The male abnormal 21 (MAB21) like proteins form a sequence related subfamily within the large and diverse family of nucleotidyltransferase (NTase) fold proteins. Here, we provide the first crystal structure of a MAB21 protein and the structure of MAB21L1 bound to CTP. MAB21L1 is a two lobed, globular protein of a mixed α/β topology with approximate molecular dimensions of 64 Å × 35 Å × 48 Å. The human MAB21L1 structure exhibits a high degree of structural conservation with cGAS but features a number of differences.

We crystallized native MAB21L1 in space group C2 with unit cell constants a = 167.7 Å, b = 177.6 Å, c = 115.6 Å, β = 126.5°. The native crystals contained 5 molecules in the asymmetric unit and diffracted to a limiting resolution of 3.05 Å. The crystal packing of MAB21L1 is unusual and consists of an intimate assembly of ten copies of MAB12L1 into a decamer, formed from two back-to-back stacked pentameric rings. The pentamer interface is composed of hydrophobic and some polar interactions between the N-terminal helix α1 of one monomer and the C-terminal helices α11 and α12 of the neighboring molecule. A citrate molecule from the crystallization condition stabilizes this interface. The citrate is coordinated by residues R344 and K340 from one monomer together with K14 and K354 from the next monomer in a very basic surface patch. During model building of the MAB21L1 structure with no nucleotides added, we observed an additional electron density not associated with the polypeptide chain in the ligand binding pocket. However, we were not able to identify by structural or mass spectrometric methods the nature of this low molecular weight ligand, which may be a buffer component or have co-purified with the protein from E. coli. The fact that the structure of MAB21L1 without any nucleotides added shows density for an unidentified molecule in the ligand binding pocket may support the suggestion that this positively-charged site acts as a binding site for an acidic ligand. Although the equivalent region of MAB21L1 is ordered in our crystal structure, it notably does not adopt the α-helical NB-loop conformation.

>[5x]GAMDIAAQAKLVYHLNKYYNEKCQARKAAIAKTIREVCKVVSDVLKEVEVQEPRFISSLNEMDNRYEGLEVISPTEFEVVLYLNQMGVFNFVDDGSLPGCAVLKLSDGRKRSMSLWVEFITASGYLSARKIRSRFQTLVAQAVDKCSYRDVVKMVADTSEVKLRIRDRYVVQITPAFKCTGIWPRSAAHWPLPHIPWPGPNRVAEVKAEGFNLLSKECHSLAGKQSSAESDAWVLQFAEAENRLQMGGCRKKCLSILKTLRDRHLELPGQPLNNYHMKTLVSYECEKHPRESDWDESCLGDRLNGILLQLISCLQCRRCPHYFLPNLDLFQGKPHSALENAAKQTWRLAREILTNPKSLEKL>[4x]AAAAKPNNLSLVVHGPGDLRLENYPIPEPGPNEVLLRMHSVGICGSDVHYWEYGRIGNFIVKKPMVLGHEASGTVEKVGSSVKHLKPGDRVAIEPGAPRENDEFCKMGRYNLSPSIFFCATPPDDGNLCRFYKHNAAFCYKLPDNVTFEEGALIEPLSVGIHACRRGGVTLGHKVLVCGAGPIGMVTLLVAKAMGAAQVVVTDLSATRLSKAKEIGADLVLQISKESPQEI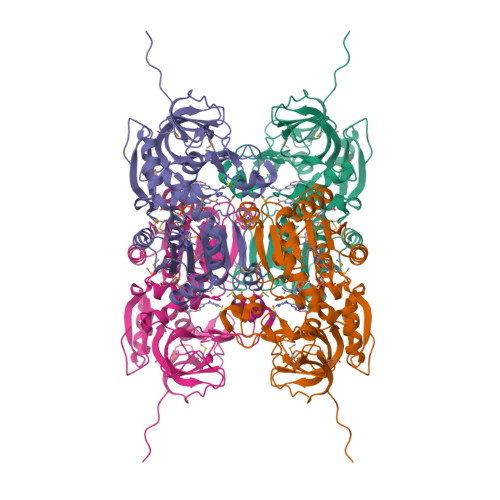ARKVEGQLGCKPEVTIECTGAEASIQAGIYATRSGGTLVLVGLGSEMTTVPLLHAAIREVDIKGVFRYCNTWPVAISMLASKSVNVKPLVTHRFPLEKALEAFETFKKGLGLKIMLKCDPSDQNP>[4x]SSNDNIELVDFQNIMFYGDAEVGDNQQPFTFILDTGSANLWVPSVKCTTAGCLTKHLYDSSKSRTYEKDGTKVEMNYVSGTVSGFFSKDLVTVGNLSLPYKFIEVIDTNGFEPTYTASTFDGILGLGWKDLSIGSVDPIVVELKNQNKIENALFTFYLPVHDKHTGFLTIGGIEERFYEGPL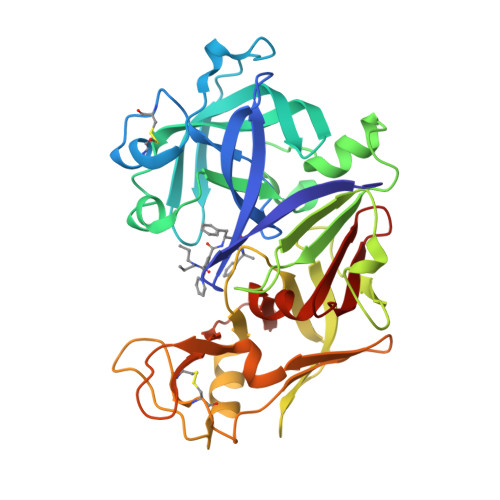TYEKLNHDLYWQITLDAHVGNISLEKANCIVDSGTSAITVPTDFLNKMLQNLDVIKVPFLPFYVTLCNNSKLPTFEFTSENGKYTLEPEYYLQHIEDVGPGLCMLNIIGLDFPVPTFILGDPFMRKYFTVFDYDNHSVGIALAKKNL>QAMEGNGPAAVHYQPASPPRDACVYSSCYSEENVWKLCEYIKNHDQYPLEECYAVFISNERKMIPIWKQQARPGDGPVIWDYHVVLLHVSSGGQSFIYDLDTVLPFPCLFDTYVEDAIKSDDDIHPQFRRKFRVICADSYLKNFASDRSHMKDSSGNWRE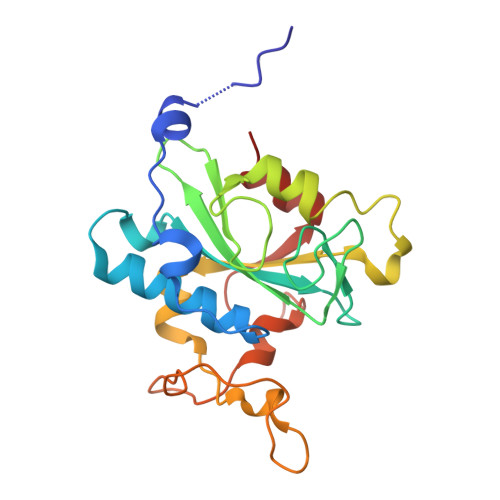PPPPYPCIETGDSKMNLNDFISMDPKVGWGAVYTLSEFTHRFGS[2x]> MHEQLSPRDQELEARLVELETRLSFQEQALTELSEALADA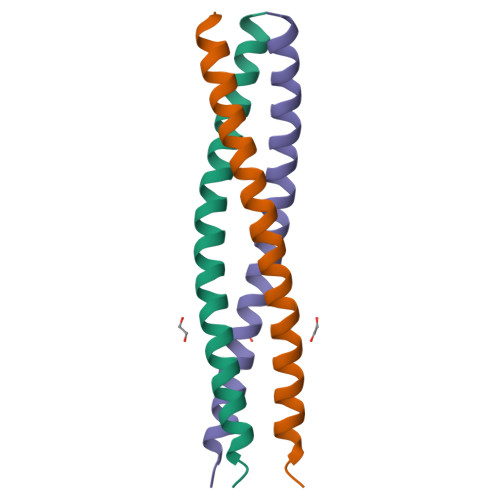RLTGARNAELIRHLLEDLGKVRSTLFADAADEPPPPHY>GAGAGAPLKKIPKRLAAILEVKPVGDVGGGVTGLLNDASEIVAWTVSAGIKHLMLYDYDGILQRNVPELRMEIHSNLAKYFGPAHVPNYAVKIPHSNKIFYNLDGIETETDVGNEIEANQEKDKIAIEISLLSNRDGRETIVDLTKTMAELAAVNELSVSDITMDLVDSELKQLVGPEPDLLLYFGPSLDLQGFPPWHIRLTEFYWEKDNNEVIYSVFIRGLRQYAGCK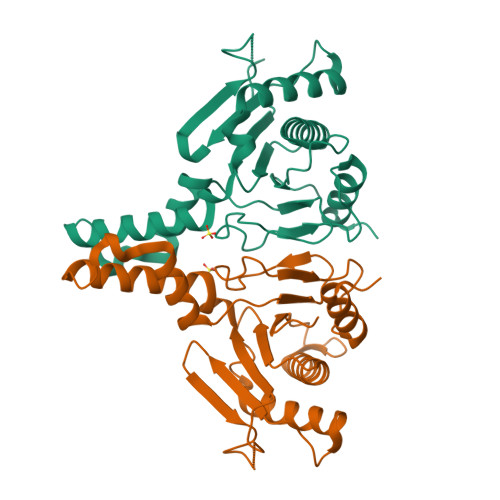VNVGK[2x]> MRID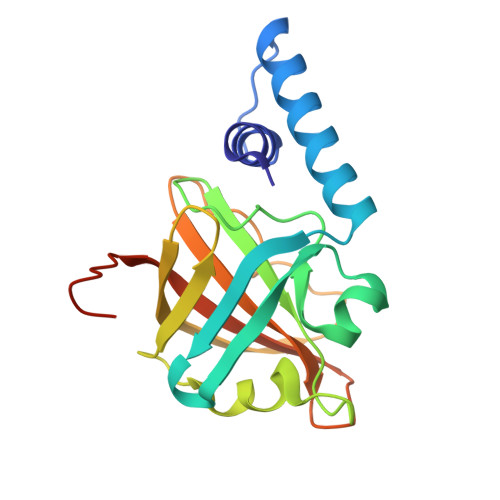LAQAFNESLNNVVSEDPYTKSRHEAGRVEYARMLELHEKIGYVEIPKIEVKLPVYAGTSETVLQKGVGHLEGTSLPIGGSDTHTVLTAHTGLPKARLFTDLTKVKIGDTFYIHNIVETLAYEVDQIVVAEPTQFEELLVKPGQDYATLLTCTPYMVNTHRLLVRGHRIPYVAEEHLEHHHHHH> TCTCCTAGG;> CUA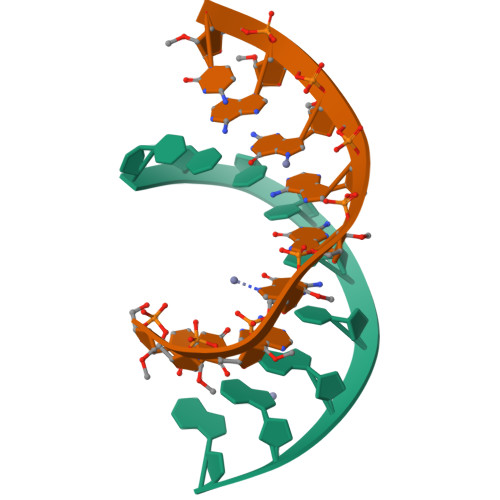GGAGAC ICV, however, has only one major surface glycoprotein, the hemagglutinin-esterase-fusion (HEF) protein, which possesses all-in-one of receptor binding, receptor destroying and membrane fusion activities. To further evaluate the infectivity and transmissibility of IDV, we expressed and purified the ectodomain of D/OK HEF, and determined that it also uses 9-O-Acetyl-Sia as its receptor by glycan microarray. We also solved the crystal structure of D/OK HEF, both in its native state (resolution of 2.4 Å) and in complex with its receptor analogue (resolution of 3.1 Å), and the structure of the enzymatically inactive HEF (resolution of 2.4 Å) alone and in complex with two receptor analogs respectively (both resolutions of 2.2 Å). Indeed, our results show that IDV HEF is functionally and structurally similar to ICV HEF, but with some distinct characteristics.

In order to study the molecular basis of IDV HEF and its receptor / substrate binding mode we solved the native X-ray crystallography structures of wild type and mutant HEFs both at a resolution of 2.4 Å. Due to the presence of cacodylate buffer in the crystallization conditions, S57 in our IDV HEF structure is covalently modified by the addition of a dimethylarsenic group. The covalent modification of active site serine by arsenic was first reported by Ian Wilson’s group in 2003, when they solved the structure of an acetyl esterase, HerE, and its complex with the inhibitor dimethylarsinic acid, and illustrated the mechanism of the broad scope inhibition of serine hydrolases by As(V)-containing organic compounds. The electron density of the covalent modification of S57 is shown in Fig 9B. In our IDV HEF structure, IDV HEF is proteolytically cleaved into the subunits HEF1 and HEF2. To confirm the proteolytic processing, we isolated IDV HEF crystals and checked for HEF2 band both by SDS-PAGE and western blot with an antibody recognizing the hexa-His tag engineered at the C terminus. Furthermore, N-terminal amino acid sequencing of the HEF2 band revealed that the first five amino acids of HEF2 were IFGID, the same with ICV HEF. The exposed fusion peptide has also been observed previously in the HEF protein of ICV and in the cleavage site of IDV HEF structure. Unambiguous electron density was seen from the ninth residue (F9) of the fusion peptide. Although we cannot observe the first eight residues in the structure, different orientations of F9 in the HEF structure and other known cleaved HA structures helped to confirm that the fusion peptide does not insert into the cavity.

>ELICIVQRVNESFSLHSGFGGNVYSMKTEPMTGFTNVTKGASVINQKDWIGFGDSRTDLTNDQFPASSDVPLAVAKKFRSLSGASLMLSAFGPPGKVDYLYQGCGKEKVFYEGVNWSPEAGIDCFGSNWTQTKKDFYSRIYEAARSSTCMTLVNSLDTKISSTTATAGTASSCSSSWMKSPLWYAESSVNPGAKPQVCGTEQSATFTLPTSFGIYKCNKHVVQLCYFVYENKAKFNTFGCGDYYQNYYDGNGNLIGGMDNRVAAYRGIANAGVKIECPSKILNPGTYSIKSTPRFLLVPKRSYCFDTDGGYPIQVVQSEWSASRRSDNATEEACLQTEGCIFIKKTTPYVGEADDNHGDIEMRQLLSGLGNNDTVCVSQSGYTKGETPFVKDYLSPPKYGRCQLKTDSGRIPTLPSGLIIPQAGTDS[2x];>IFGIDDLIFGLLFVGFVAGGVAGGYFWGRSNGGGGGASVSSTQAGFDKIGKDIQQLRNDTNAAIEGFNGRIAHDEQAIKNLAKEIEDARAEALVGELGIIRSLIVANISMNLKESLYELANQITKRGGGIAQEAGPGCWYVDSENCDASCKEYIFNFNGSATVPTL[2x]>[2x]MSKPSIVILGAGYGGIVAALGLQKRLNYNEADITLVNKNDYHYITTELHQPAAGTMHHDQARVGIKELIDEKKIKFVKDTVVAIDREQQKVTLQNGELHYDYLVVGLGSEPETFGIEGLREHAFSINSINSVRIIRQHIEYQFAKFAAEPERTDYLTIVVGGAEFTGIEFVGELADRMPELCAEYDVDPKLVRIINVEAAPTVLPGFDPALVNYAMDVLGGKGVEFKIGTPIKRCTPEGVVIEVDGEEEEIKAATVVWTGGVRGNSIVEKSGFETMRGRIKVDPYLRAPGHENIFIVGDCALIINEENNRPYPPTAQIAIQHGENVAANLAALIRGGSMTPFKPHIRGTVASLGRNDAIGIVGGRKVYGHAASWLKKLIDMRYLYLIGGLSLVLKKGRFHHHHHH

Type-II NADH:quinone oxidoreductase (NADH dehydrogenase-2, NDH-2) is a membrane-bound dehydrogenase that oxidizes NADH and reduces quinones and is a central feature of the respiratory chain in many diverse species, but not in animals. NDH-2 is also much smaller and simpler in structure than complex I – it comprises only a single subunit and one flavin redox cofactor. All of them are homodimers, with each monomer containing two Rossmann folds that form nucleotide-binding sites for a noncovalently bound flavin adenine dinucleotide (FAD) and the NADH substrate. Our study has revealed how the NADH:quinone oxidoreduction reaction proceeds in two half reactions (NADH oxidation + reduction of the flavin, and re-oxidation of the flavin + reduction of quinone) that occur independently of each other and use spatially distinct substrate-binding sites.

To test the proposal that the two substrate reactions are independent of each other we mutated a key residue in each substrate-binding site. G164 is positioned next to the adenine-proximal ribose of the bound nucleotide and I379 is positioned at the entry to the quinone-binding pocket. Structures of the two mutants, at 3.2 and 2.7 Å resolution, respectively, confirmed that the structural changes are localized and the integrities of the structures are maintained. G164E crystallized in a different space group (P41212) to the wild-type (WT) protein, but the glutamate side chain could be observed confidently in only one of two molecules in the asymmetric unit. In comparison with WT, G164E and I379E exhibit RMSD values of 0.54 Å (Cα of 395 residues) and 0.45 Å (Cα of 393 residues), respectively, with no substantial additional differences. For the G164E variant the KM for NADH increases drastically to more than 1 mM, consistent with the mutation compromising NADH binding. Furthermore, the observed rates drop drastically (only ~1% of the WT activity is observed in even 600 μM NADH), and, as a consequence, the apparent KM value for menadione decreases significantly because the turnover rate is ‘capped’ by the slow rate of NADH oxidation. Subsequent additions of NAD+ to the reduced protein also failed to produce a CTC. Figure 6C shows that the reaction between G164E and NADH is very slow (~0.2 s−1 in 2 μM NADH), similar to the reaction of the WT with NADPH (~0.3 s−1 in 2 μM NADPH), consistent with weak nucleotide binding. Conversely, when NADH-reduced G164E was reacted with menadione rapid oxidation of the flavin (~175 s−1 in 1.5 μM menadione, matching the ~200 s−1 rate for WT) was observed, demonstrating that the quinone-binding site is fully functional, irrespective of the functionality of the NADH-binding site.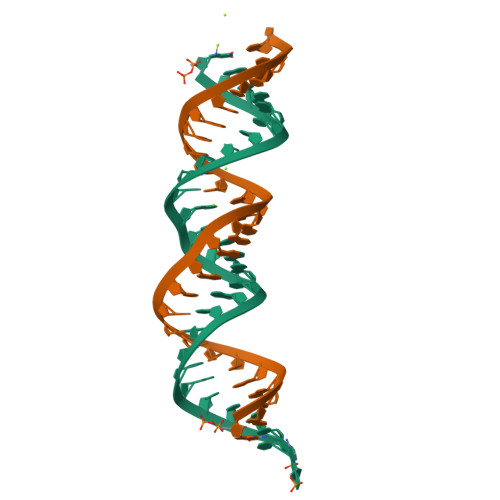>GGUGACCUCCCGGGAGCGGGGGACCACUA[3x]> GEESRNTTVLDTTTTLQSSGFGRAFFGEAFNDLKTLMRRYQLYGQLLLSVTTDKDIDHCMFTFPCLPQGLALDIGSAGSPHEIFNRCRDGIIPLIASGYRFYRGDLRYKIVFPSNVNSNIWVQHRPDRRLEGWSAAKIVNCDAVSTGQGVYNHGYASHIQITRVNN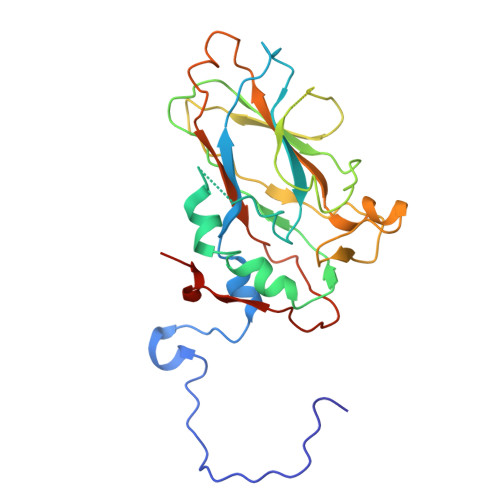VIELEVPFYNATCYNYLQAFNASSAASSYAVSLGEISVGFQATSDDIASIVNKPVTIYYSIGDGMQFSQWVGYQPMMILDQLPAPVVRAVPE>[2x]MTQVAEIKSPHEQRLEDNIAGKEDIYRESHKRVFKLLERFDGQKPAIDVERALYFTQSMAETVGQPLVLRWAKALMNVAKNITVMVQDDQLLLGRCGGHDGRYGILYPELDGDFLDIAVRDLPTRPQSPASISPEDAKIVVEQIAPFWKGRTYHEALNKALPAEVHKLTYDDPDGLISRFIVNETSSFRSSIQWVHDYEVVLKRGFNGLKQEMEEKLAALDPASPVDQVDKRPFIEATILVCDAIVLWAKRHADAARKAAEACADPVRKAELIRMAENAEHVPANPARDFYEAVQSQYFTQMFSRLEQKTGTTISNGRMDQYFYPFYKKDMEAGILTDEKTLEYLECMWVGMAEFIDMYISPAGGAFNEGYAHWEAVTIGGQTPDGRDATNDLTYLFLKSKREFPLHYPDLAARIHSRAPERYLWDVAETIKFGSGFPKLCNDEECIPLYVSKGATFEEALDYAVSGCIEIRMPNRDTYTSGGAYTNFASAVEMALYDGKMKKYGDVQLGIQTGDARKFKSWDEFWNAYVQQHMLLLRTTFIQQYIVIQTRAKHFAQPMGSVLHALCRKHCIDLHQPQIPEGLNFGYFEFMGLGTVIDSLAAIKKLVFEDKKLTMDQLIDALEANFEGYEDIQQLLRTAPCYGNDDEYADEIGRELDRMAVSFAAKYGKEMGINNDARYVPFTSHVPFGKVVSATPNGRVAWFPLADGSSPSHGADHNGPTAILLSNHNTKNYGMRARAARLINVKFTPKCVEGDAGTEKLVQFIRTWCDLKLWHIQFNVINADTLKKAQKDPQKYRNLIVRIAGYSAYFVDLTPDLQNDLIARTGHDQM

Desulfonation of isethionate by the bacterial glycyl radical enzyme (GRE) isethionate sulfite-lyase (IslA) generates sulfite, a substrate for respiration that in turn produces the disease-associated metabolite hydrogen sulfide. IslA belongs to the glycyl radical enzyme (GRE) superfamily, which performs diverse chemical reactions under anaerobic conditions (Backman et al., 2017). As is the case for the core architecture of all characterized GRE eliminases (Backman et al., 2017), IslA is dimeric with each monomer having a buried active site located centrally within a barrel comprised of two five-stranded half β barrels, anti-parallel to each other (β1–10), and surrounded by α helices. Gly805 and Cys468 are 5.2 Å from each other, competent for radical transfer from Gly805 to Cys468, and for the generation of a transient thiyl radical that initiates catalysis on the substrate.

During model refinement, positive difference density was observed in the active site that resembled glycerol, a component of the purification buffer and cryoprotectant. Due to the buried nature of the active site, substrate access channels and product release channels are required. To investigate whether other GREs have a similar channel to that of BSS, we ran an analysis of available GRE structures using the program CAVER 3.0 (Chovancova et al., 2012) and compared channels identified with the toluene channel of BSS. We find an equivalent channel to that in BSS in the two glycerol-bound structures of HypD and IslA. The lengths of these channels range between 14 and 19 Å from the active site to the protein surface. Residues along the channels are highly conserved in each of these four GREs, consistent with these channels playing a functional role. The products, acetaldehyde and sulfite, are released, potentially through a highly conserved channel seen in IslA and other GREs, allowing for the next Ise substrate to bind.> MSLKHVVVIGAVALGPKAACRFKRLDPEAHVTMIDQASRISYGGCGIPYYVSGEVSNIESLQATPYNVVRDPEFFRINKDVEALVETRAHAIDRAAHTVEIENLRTGERRTLKYDKLVLALGSKANRPPVEGMDLAGVTPVTNLDEAEFVQHAISAGEVSKAVIVGGGFIGLEMAVSLADMWGIDTTVVELADQIMPGFTSKSLSQMLRHDLEKNDVVVHTGEKVVRLEGENGKVARVITDKRTLDADLVILAAGVSPNTQLARDAGLELDPRGAIIVDTRMRTSDPDIFAGGDCVTIPNLVTGKPGFFPLGSMANRQGRVIGTNLADGDATFPGAVGSWAVKLFEGSASGAGLTVEGALREGYDAVNVHVEQFDRAHFYPEKTIMTLQLVVDRPTRRVLGIQGFSTLGDALTARINAVATMLASKPTVEDISNAEVVYSPPFASAMDIV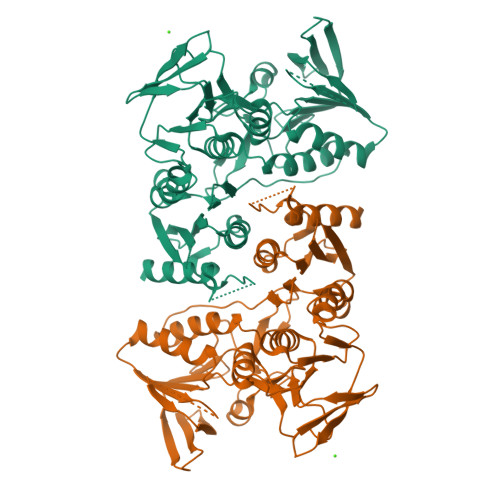NVAGNVADNVLAGREGHHHHHH> GSHMAATAAEAVASGSGEPREEAGALGPAWDESQLRSYSFPTRPIPRLSQSDPRAEELIENEEPVVLTDTNLVYPALKWDLEYLQENIGNGDFSVYSASTHKFLYYDEKKMANFQNFKPRSNREEMKFHEFVEKLQDIQQRGGEERLYLQQTLNDTVGRKIVMDFLGFNWNWINKQQGKRGWGQLTSNLLLIGMEGNVTPAHYDEQQNFFAQIKGYKRCILFPPDQFECLYPYPVHHPCDRQSQVDFDNPDYERFPNFQNVVGYETVVGPGDVLYIPMYWWH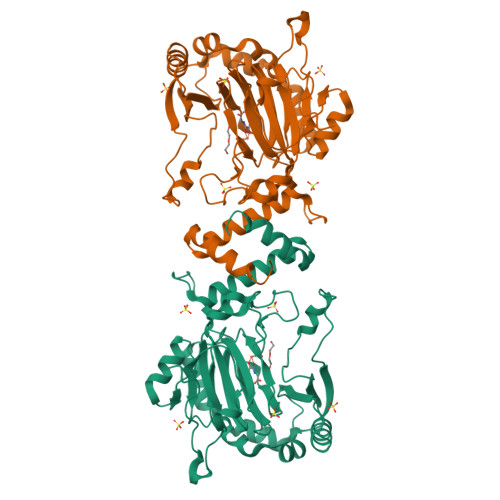HIESLLNGGITITVNFWYKGAPTPKRIEYPLKAHQKVAIMRNIEKMLGEALGNPQEVGPLLNTMIKGRYN>PATGEKKECWSWESYLEEQKAITAPVSLFQDSQAVTHNKNGFKLGMKLEGIDPQHPSMYFILTVAEVCGYRLRLHFDGYSECHDFWVNANSPDIHPAGWFEKTGHKLQPPKGYKEEEFSWSQYLRSTRAQAAPKHLFVSQSHSPPPLGFQVGMKLEAVDRMNPSLVCVASVTDVVDSRFLVHFDNWDDTYDYWCDPSSPYIHPVGWCQKQGKPLTPPQDYPDPDNFCWEKYLEETGASAVPTWAFKV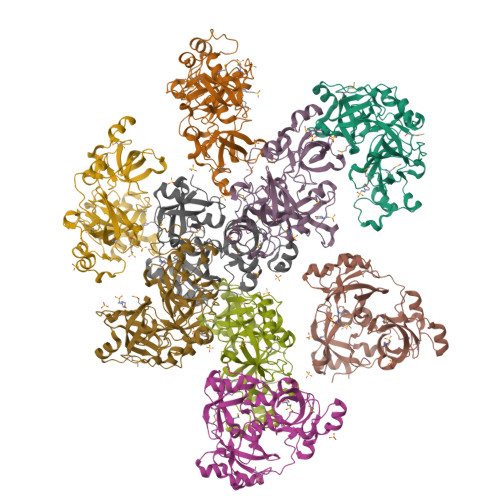RPPHSFLVNMKLEAVDRRNPALIRVASVEDVEDHRIKIHFDGWSHGYDFWIDADHPDIHPAGWCSKTGHPLQPPLGPREPSSAS[3x]> SAEGTRQSPINIQWKDSVYDPQLAPLRVSYDAASCRYLWNTGHAFQVEFDDSCEDSGISGGPLGNHYRLKQFHFHWGATDEWGSEHAVDGHTYPAELHLVHWNSTKYENYKKASVGENGLAVIGVFLKLGAHHQALQKLVDVLPEVRHKDTQVAMGDFDPSCLMPACRDYWTYPGSLTTPPLAESVTWIVQKTPVEVSPS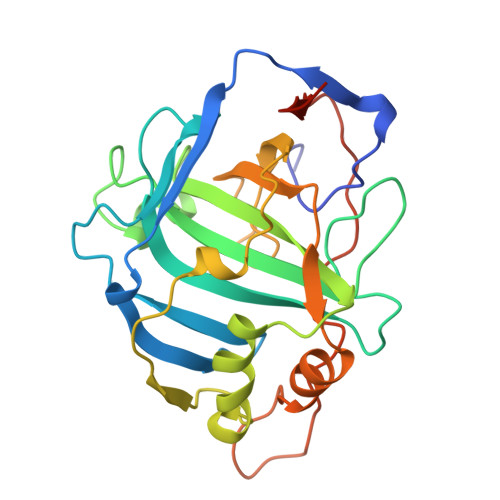QLSMFRTLLFSGRGEEEDVMVNNYRPLQPLRDRKLRSSFRLDRTKMRS>GSMQYFAQIVNREENKWPSEPINKYIHMIWIGPKNISDKNIRLSLQTAQKNPDYSTTIIYDSGISGYEAARNFMSEKFKASKITLVDIRNKGYFHQLQQEPSFTYYEEVIRNKKFAQASDILRLLVLKYEGGIYKDIDDIQIKGFGSLAFPKGIGVMREYVPEAGKSAAFPNSPIAATKNNPVVNKTLELAVENYRHGEKNVLKLAGPDVFTKALYQEIPGMCSQVLGTQLEQFELAKRQALKMPLEKPKSFIDEQLTLQEKAKISRPYKAIRGLSEYVCNGADHSWATDMLGSSTKMY[2x]

The respective glycosyltransferases are important virulence factors such as the Clostridioides difficile toxins A and B. Here, we describe two glycosyltransferases of Yersinia species that have a high sequence identity: YeGT from the zoonotic pathogen Yersinia enterocolitica and YkGT from the murine pathogen Yersinia kristensenii. We show that both modify Rho family proteins by attachment of GlcNAc at tyrosine residues (Tyr-34 in RhoA). sYeGT has a cone-shaped structure comprised of a globular domain with a Rossmann-like fold on top of a three-helix bundle. The catalytically active domain is the Rossmann-like fold domain, which features a 6-stranded antiparallel β-sheet flanked by 7 α-helices.

Interestingly, in the absence of ligands, sYeGT crystals belonging to space group P43212 appeared rapidly and diffracted X-rays up to 2.3-Å resolution while in the presence of UDP-GlcNAc, P21 crystals were visible only after 8 weeks but diffracted better, with a resolution up to 1.12 Å. The asymmetric unit of the ligand bound sYeGT crystal comprises two molecules. Each protomer includes the complete N-terminal part of the construct but lacks 14 residues at the C-terminal end. Although sYeGT was crystallized in the presence of the substrate UDP-GlcNAc and Mn+2, only the UDP moiety was visible in the electron density map suggesting that the sugar nucleotide had been hydrolyzed during the crystallization process. The uracil moiety is mainly stabilized by residues from the WIG-motif (residues 44–46). In detail, Trp-44 forms a stacking interaction with the purine base, and backbone atoms of Ile-45 and Lys-48 form hydrogen bonds with the polar side of the base. The ribose moiety is stabilized by hydrogen bonds to main chain atoms from residues Ile-43 and Ile-151 and to the gamma-oxygen from Ser-133. The manganese ion is coordinated on one side by the pyrophosphate moiety of UDP and on the other side by the carboxylic groups of Asp-150 and Asp-152, the residues of the DxD motif. Notably, a third aspartate residue, Asp-153, is indirectly involved in the manganese coordination via a water molecule. Another notable feature is the loop flanking the nucleotide binding site (loop F, residues 171–188), which is bent toward the nucleotide when the latter is present.>AAAAANHSTQESGFDYEGLIDSELQKKRLDKSYRYFNNINRLAKEFPLAHRQREADKVTVWCSNDYLALSKHPEVLDAMHKTIDKYGCGAGGTRNIAGHNIPTLNLEAELATLHKKEGALVFSSCYVANDAVLSLLGQKMKDLVIFSDELNHASMIVGIKHANVKKHIFKHNDLNELEQLLQSYPKSVPKLIAFESVYSMAGSVADIEKICDLADKYGALTFLDEVHAVGLYGPHGAGVAEHCDFESHRASGIATPKTNDKGGAKTVMDRVDMITGTLGKSFGSVGGYVAASRKLIDWFRSFAPGFIFTTTLPPSVMAGATAAIRYQRCHIDLRTSQQKHTMYVKKAFHELGIPVIPNPSHIVPVLIGNADLAKQASDILINKHQIYVQAINFPTVARGTERLRITPTPGHTNDLSDILINAVDDVFNELQLPRVRDWESQGGLLGVGESGFVEESNLWTSSQLSLTNDDLNPNV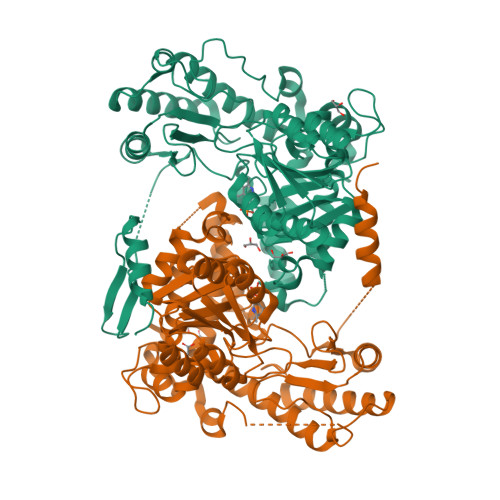RD[2x]>GHMRRVVITGLGIVSCLGNDKDTVSANLRAGRPGIRFNPSYAEMGLRSHVSGSVDLNLEELIDRKVFRFMGDAAAYAYLAMEQAIKDSGLTPEQISNPRTGLIAGSGGASTLNQMEAIDTLREKGVKRIGPYRVTRTMGSTVSACLATPFQIKGVNYSISSAAATSAHCIGQAMEQIQLGKQDVVFAGGGEEEHWSQSCLFDAMGALSTQYNETPEKASRAYDAKRDGFVIAGGGGMVVVEELEHALKRGAKIYAEIVGYGATSDGYDMVAPSGEGAIRCMQQALATVDAPIDYLNTHGTSTPVGDVAEIRGVREVFGDKAPAISSTKSLSGHSLGAAG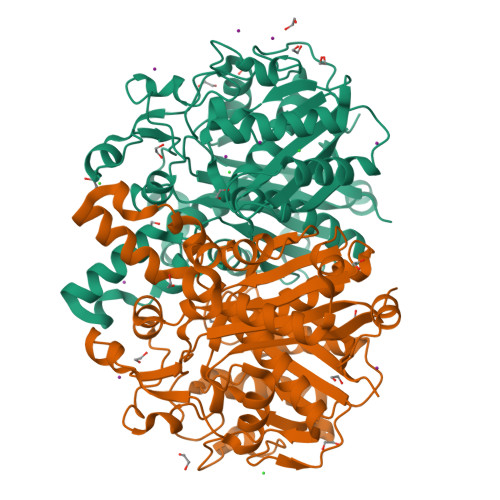VHEAIYCLLMMEGGFIAGSANIDELDPEVADLPILRETRENAKLDTVMSNSFGFGGTNATLVLKRWQG[2x]>[4x]GQNHHEVVKFMDVYQRSYCHPIETLVDIFQEYPDEIEYIFKP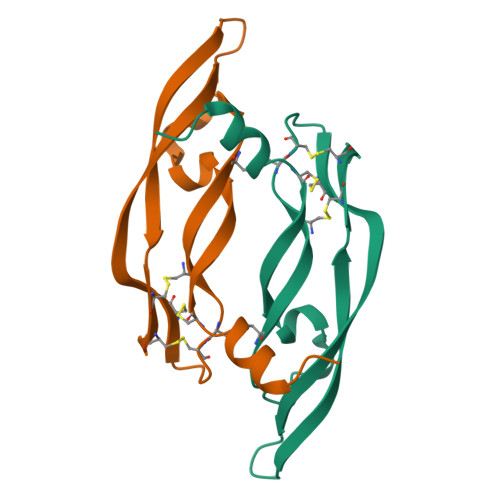SCVPLMRCGGCCNDEGLECVPTEESNITMQIMRIKPHQGQHIGEMSFLQHNKCECRPKKD METHYL ARACHIDONYL FLUOROPHOSPHONATE | C21 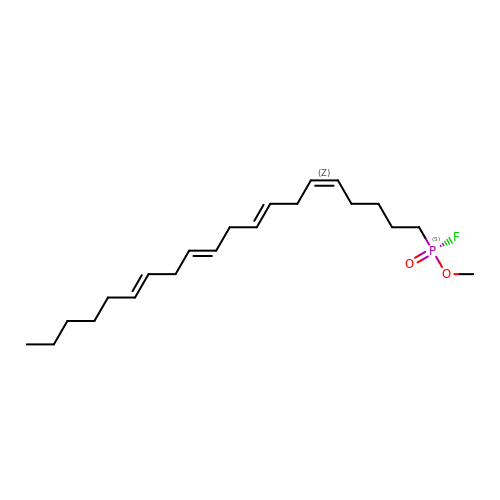H36 F O2 P | KWKZCGMJGHHOKJ-WTIHWRCNSA-N> GLFSQIELSFSASNLRDRDVLSKSDPMVVVYQKEKDATLSEVFRSEVVLNSLAPKWIKKFIVAYHFETVQTLVFRVYDVDTKFQNSREEMLKLDEQQFLGEATCALSEIITKSTRTSTLELKRKDGFAPQAQPHHGKLIIHAEESLASKISTEIVFRCSNLESKDLFSKSDPFLVVSKIVEHGTPIPVSKTEVRKNDLNPIWKPVFLSV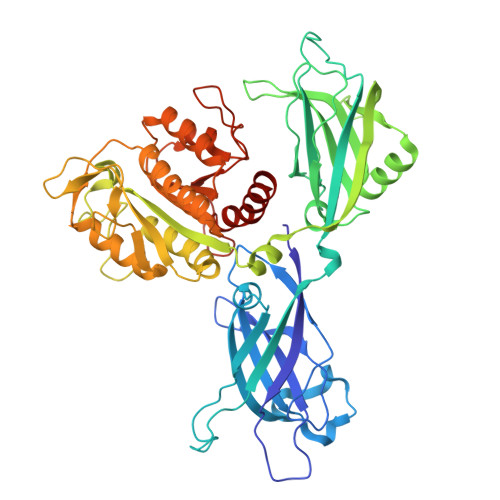QQVGSKDSPVIIECSDFNSNGKHSLIGKVQKSLSDLEKLHLAGQGINFSLPTGAGQNKVLKSQLFVDKFTETVHHTFLEYLASGFELNFMVAIDFTASNGNPRLPDSLHYIDPSGRLNAYQRAIMDVGEVLQFYDSDKRFPAWGFGARPIDAPVSHCFNLNGSSSYSEVDGIQGIMTSYTSALFNVSLAGPTLFGPVINAAAMIASASLAQGSRKYYVLLIITDGVITDLQETKDALVSASDLPLSILIVGVGGADFKEMEILDADKGERLESSSGRLASRDIVQFVALRDVQYGEISVVQALLAELPSQFLTYMRIRN>[2x]MVLYFIGLGLYDERDITVKGLECAKKCDYVFAEFYTSLMAGTTLGRIQKLIGKEIRVLSREDVELNFENIVLPLAKENDVAFLTPGDPLVATTHAELRIRAKRAGVESYVIHAPSIYSAVGITGLHIYKFGKSATVAYPEGNWFPTSYYDVIKENAERGLHTLLFLDIKAEKRMYMTANEAMELLLKVEDMK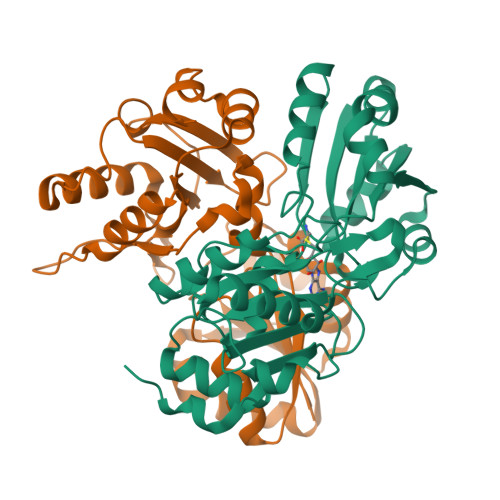KGGVFTDDTLVVVLARAGSLNPTIRAGYVKDLIREDFGDPPHILIVPGKLHIVEAEYLVEIAGAPREILRVNV> MKIVYWSGTGNTEKMAELIAKGIIESGKDVNTINVSDVNIDELLNEDILILGCSAMNDEVLEESEFEPFIEEISTKISGKKVALFGSYGWGD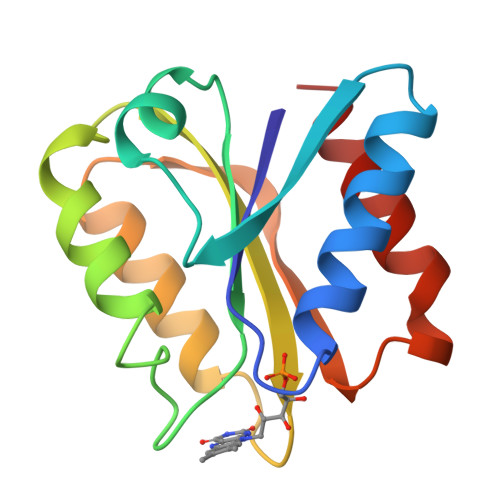GKWMRDFEERMNGYGCVVVETPLIVQNEPDEAEQDCIEFGKKIANI>MGADDVVDSSKSFVMENFSSYHGTKPGYVDSIQKGIQKPKSGTQGNYDDDWEGFYSTDNKYDAAGYSVDNENPLSGKAGGVVKVTYPGLTKVLALKVDNAETIKKELGLSLTEPLMEQVGTEEFIKRFGDGASRVVLSLPFAEGSSSVKYINNWEQAKALSVELEINFETRGKRGQDAMYEYMAQACAGNRVRRSVGSSLSCINLDWDVIRDKTKTKIESLKEHGPIKNKMSESPNKTVSEE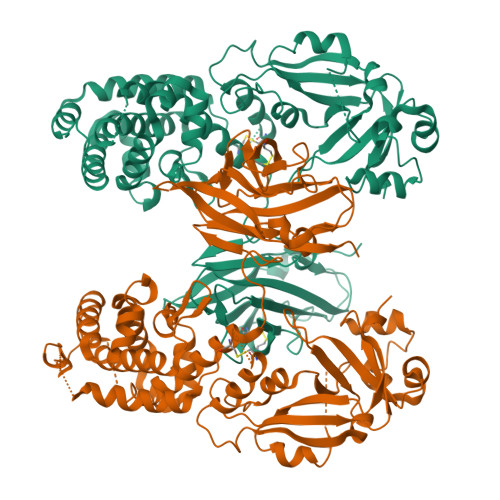KAKQYLEEFHQTALEHPELSELKTVTGTNPVFAGANYAAWAVNVAQVIDSETADNLEKTTAALSILPGIGSVMGIADGAVHHNTEEIVAQSIALSSLMVAQAIPLVGELVDIGFAAYNFVESIINLFQVVHNSYNRPAYSPGHKTQPFLHDGYAVSWNTVEDSIIRTGFQGESGHDIKITAENTPLPIAGVLLPTIPGKLDVNKSKTHISVNGRKIRMRCRAIDGDVTFCRPKSPVYVGNGVHANLHVAFHRSSSEKIHSNEISSDSIGVLGYQKTVDHTKVNSKLSLFFEIKSMA[2x]D-LIMONENE 1,2-EPOXIDE | C10 H16 O | 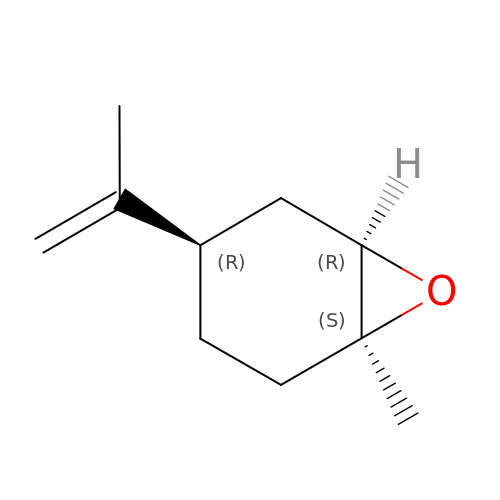CCEFMUBVSUDRLG-BBBLOLIVSA-N>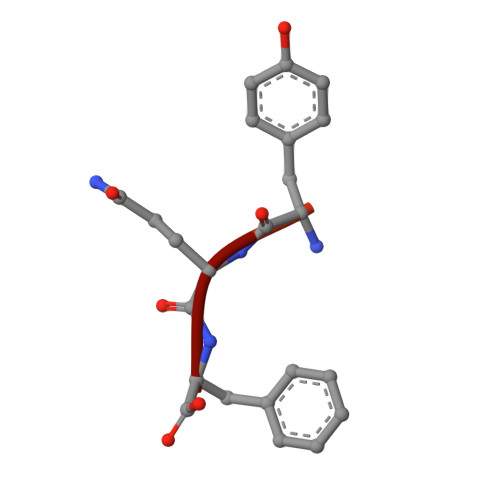 DNRLGLVYQF N-{5-[4-(2-amino-4-oxo-3,4-dihydrothieno[2,3-d]pyrimidin-6-yl)butyl]furan-2-carbonyl}-L-glutamic acid 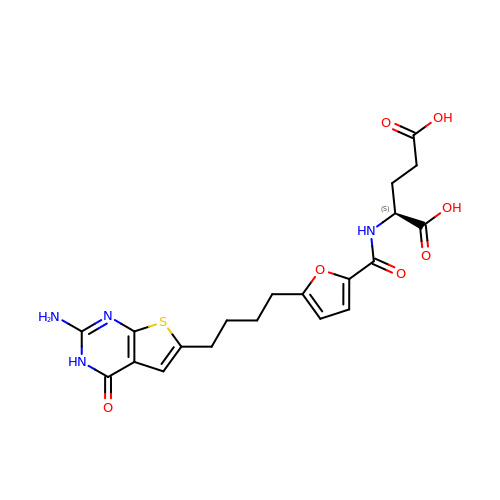| C20 H22 N4 O7 S | LYDGQYDYRQVOBF-ZDUSSCGKSA-N>MSKSKVDNQFYSVEVGDSTFTVLKRYQNLKPIGSGAQGIVCAAYDAVLDRNVAIKKL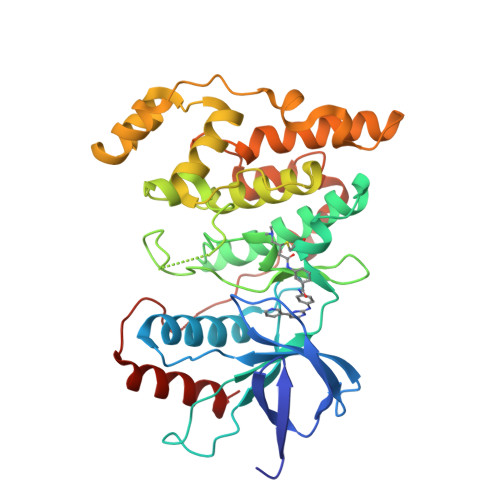SRPFQNQTHAKRAYRELVLMKCVNHKNIISLLNVFTPQKTLEEFQDVYLVMELMDANLCQVIQMELDHERMSYLLYQMLCGIKHLHSAGIIHRDLKPSNIVVKSDCTLKILDFGLARTAGTSFMMTPYVVTRYYRAPEVILGMGYKENVDIWSVGCIMGEMVRHKILFPGRDYIDQWNKVIEQLGTPCPEFMKKLQPTVRNYVENRPKYAGLTFPKLFPDSLFPADSEHNKLKASQARDLLSKMLVIDPAKRISVDDALQHPYINVWYDPAEVEAPPPQIYDKQLDEREHTIEEWKELIYKEVMNSE[2x]>[2x]MKLYETAMTPSCKRVSIFLKEIGGEVERVALNVR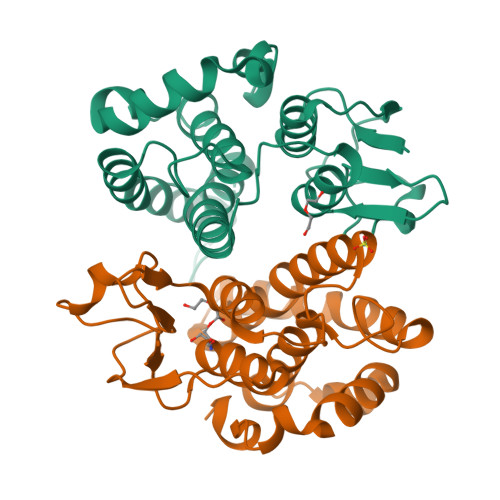EGDNLSESFKQKSVNGKVPLLELDDGTTICESVAICRYLDEAFENDLALFGANQLERAQVEMWHRVVEFQGLYAAFQAFRNITAIYQDRENCVAAWGEESKSRVLEFLPTLDTRLSESEYIATDQFSVVDITGYIFIGFAVNGLSIEVFEKYPNIARWFEQVSARDAFQSSGLEVLFQ> MDSKHQCVKLNDGHFMPVLGFGTYAPPEVPRSKALEVTKLAIEAGFRHIDSAHLYNNEEQVGLAIRSKIADGSVKREDIFYTSKLWSTFHRPELVRPALENSLKKAQLDYVDLYLIHSPMSLKPGEELSPTDENGKVIFDIVDLCTTWEAMEKCKDAGLAKSIGVSNFNRRQLEMILNKPGLKYKPVCNQVECHPYFNRSKLLDFCKSKDIVLVAYSALGSQRDKRFVDPNSPVLLEDPVLCALAKKHKRTPALIALRYQLQRGVVVLAKSYNEQRIRQNVQVFEFQLTAEDMKAIDGLDRNLHYFNSDSFASHPNYPYSDEYLEHHHHH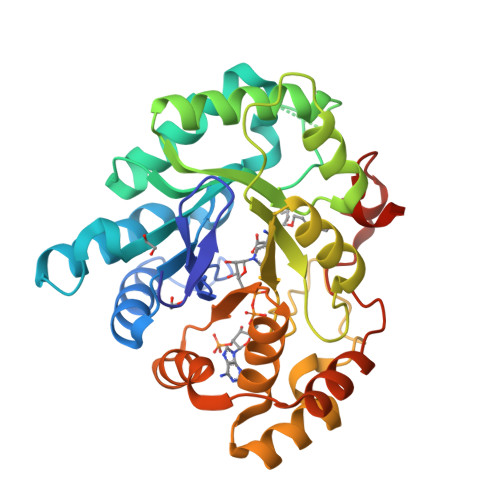H Phycobiliproteins (PBPs) and linker proteins (LPs) are mutually arranged in cyanobacteria and red algae to form multi-molecular assemblies of around 4–8 MDa called phycobilisomes (PBS). The core invariantly contains allophycocyanin (APC, absorption λmax ~653 nm) and associated LPs. The heterodimer (αβ monomer) of two homologous α- and β- subunits of PE, PC and APC proteins is the building block of PBS. The unique red-shifted absorbances of APC chromophores and their fluorescence emission overlapping to that of chlorophyll has been found to play major connecting role in this light funneling phenomenon.

In the present paper, we report the first crystal structure of APC isolated from the marine cyanobacterium, Phormidium sp. A09DM (formerly known as Lyngbya sp. A09DM). The APC crystal belonged to space group H 32, with unit-cell parameters a = b = 101.2 Å, c = 193.0 Å. Although only one αβ monomer is in the asymmetric unit, a trimer of the Phormidium protein exists in the crystal structure. The trimer in the crystals is generated by the crystallographic symmetry. The protein is observed to exist as a trimer both in solution and in crystals. The structures of α- and β- subunits are comprised of seven α-helices adopting globin-like fold (SCOP, 46457) and their folds are identical to that of other known APC structures. One PCB chromophore is covalently bonded to the conserved Cys-81 of α-subunit (α-chromophore) and other chromophore is covalently linked to conserved Cys-81 of β-subunit. Trimer formation packs the amino acid residues of β-subunit closer to α-chromophore, while atoms of β-subunit only interact with its bound chromophore. The β-subunit contributes three Tyr, three Thr and one Leu residues to the microenvironment of the α-chromophore. However, microenvironment of the PCB chromophore bound to α-subunit is enriched by hydrophobic residues, owing to the presence of Met-85 and Ala-129 residues, in the Phormidium APC protein.

> MSIVTKSIVNADAEARYLSPGELDRIKGFVTSGERRLRIAQVLTESRERIVKQAGDQLFQKRPDVVSPGGNAYGEEMTATCLRDMDYYLRLITYGVVAGDVTPIEEIGLVGVREMYNSLGTPIPAVAEAVRCMKSVASSLLSGEDAAEAASYFDYVVGAMQ;> MQDAITAVINSSDVQGKYLDGSAMEKLKAYFQTGELRVRAATTISANAAEIVKDAVAKSLLYSDITRPGGNMYTTRRYAACIRDLDYYLRYSTYAMLAGDPSILDERVLNGLKETYNSLGVPVGATVQAIQAMKEVTATLVGADAGKEMGVYFDYICSGLS> MSWWWAGAIGAAKKRSDEDEALPKHSSVALIVGVTGIVGNSLAEILPLADTPSGPWKVYGVARRPRPAWNEDNPINYIRCDISDPKDTQEKLSPLTDITHVFYVTWANRSTEVERCEANGKMLKNVLDVVIPNCPDLKHISLQTGRKHYVGPFELIGKIETHDPPFTEDLPRLKFDNFYYTQEDLLFEEVEKKEGLTWSVHRPGNIFGFSPYSMMNLVGTLCVYAAICKHEGKVLRFPGCKAAWDGYSDCSDADLIAEHHIWAAVDPYAKNEAFNVSNGDVFKWKHFWKVLAEQFGVECGEYEEGENLKLQDLMKGKEPVWEEIVRENGLASTNLEDVAVWWFSDAVLDIPCPLDSMNKSKEHGFLGFRNSKNSFISWIDKAKAYKIVP

In order to investigate the function of this protein, which we termed PmMOR (Plantago major multisubstrate oxido-reductase), we expressed, purified and determined its activity with different substrates including 8-oxogeranial, citral and 5β-progesterone. The structural studies and enzymatic assays presented here demonstrate that PmMOR is able to accommodate diverse substrates within its active site, to catalyse the reduction of aldehydes and carbon-carbon double bonds and to perform reductive cyclisation reactions to form the iridoid backbone. Each monomer of the protein folds into two domains, a Rossmann domain that binds NADP(H) and forms much of the active site cavity and a largely α-helical capping domain. The SDR superfamily generally contains a catalytic tetrad of ASN-SER-TYR-LYS or triad consisting of SER-TYR-LYS; however, the 5ß–PORs lack this canonical tetrad or triad and are thought to use only an active site TYR and LYS residue for catalysis.

In order to probe the substrate specificity determinants and enzymatic mechanism, we further solved the crystal structures of PmMOR as a ternary complex with NADP+ and 8-oxogeranial, PmMOR in complex with NAD+ and progesterone, PmMORV150M in complex with NADP+ and citral, and PmMORV150M in complex with NADP+ and progesterone. A second dataset of wild-type protein in complex with progesterone also yielded an extended difference map peak in the same region, into which progesterone could be modeled and refined, however the crystals diffracted to lower resolution and the map was of poorer quality. It is likely that the size of the pocket allows for significant movement of the ligand, and the observed density is an average of multiple conformations. Nevertheless, the binding region presented here of progesterone is largely consistent with the model suggested by Thorn et al.. and Hu et al., and places the C3 ketone in the same position as the aldehyde in our 8-oxogeranial and citral bound structures. By contrast, our data and model favor a conformation where the steroid is flipped 180° when compared to the previous models. This conformation fits the difference electron density much better as demonstrated by the higher correlation coefficients (CC with the difference map 1.75x higher for the flipped conformation) than the best fit from Thorn et al. and avoids a steric clash with ASN-205 which occludes part of the binding pocket in PmMOR. While progesterone was poorly utilized as a substrate by PmMOR based on very low specific activity, the enzyme was able to reduce progesterone to 5ß-dihydroprogesterone, even though this compound is not found in P. major and is thus not a physiological substrate. Interestingly, P. major does not have the cardenolide progesterone pathway, however the enzyme is able to accommodate this non-physiological substrate and perform the reduction reaction.>MATIIFAGRSNVGKSTLIYRLTGKKVRRGKRPGVTRKIIEIEWKNHKIIDMPGFGFMMGLPKEVQ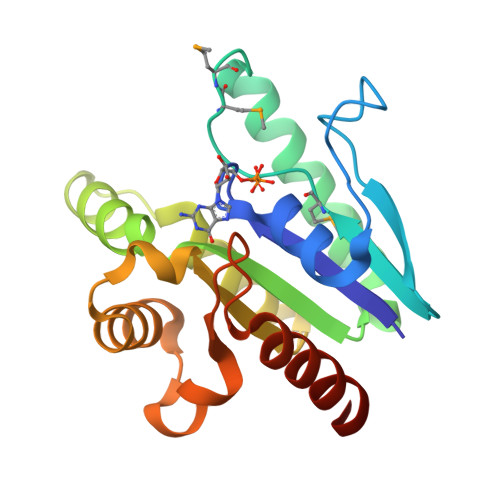ERIKDEIVHFIEDNAKNIDVAVLVVDGKAAPEIIKRWEKRGEIPIDVEFYQFLRELDIPTIVAVNKLDKIKNVQEVINFLAEKFEVPLSEIDKVFIPISAKFGDNIERLKNRIFEVIRERQGRRV[3x]>GHHHHHHHHHHSSGHIEGRHMKPSFSPRNYKALSEVQGWKQRMAAKELARQNMDLGFKLLKKLAFYNPGRNIFLSPLSISTAFSMLCLGAQDSTLDEIKQGFNFRKMPEKDLHEGFHYIIHELTQKTQDLKLSIGNTLFIDQRLQPQRKFLEDAKNFYSAETILTNFQNLEMAQKQINDFISQKTHGKINNLIENIDPGTVMLLANYIFFRARWKHEFDPNVTKEEDFFLEKNSSVKVPMMFRSGIYQVGYDDKLSCTILEIPYQKNITAIFILPDEGKLKHLEKGLQVDTFSRWKTLLSRRVVCVSVPRL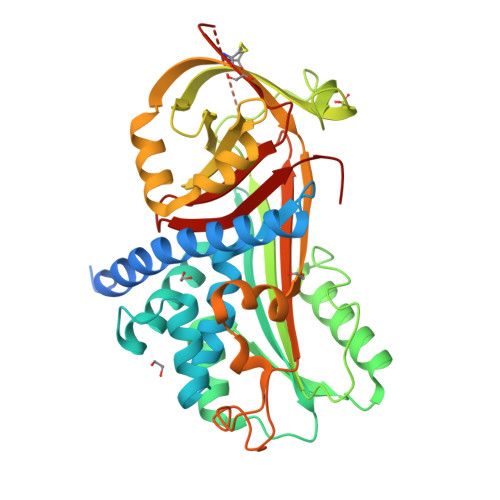HMTGTFDLKKTLSYIGVSKIFEEHGDLTKIAPHRSLKVGEAVHKAELKMDERGTEGAAGTGAQTLPMETPLCVKIDKPYLLLIYSEKIPSVLFLGKIVNPIGK[2x]>MGSSWSHPQFEKSSGLVPRGSHMLEQCPVTKIGPWGSSHEGTVQDITESPKRLESITLYHGWSVDSISFTYLDHAGEKHKAGPWGGPGGDPIMIEFGSSEFLKEVSGTFGPYEGSTVITSINFITNKQTYGPFGRQEGTPFSVPAQNNSSIVGFFGRSGKYINAVGV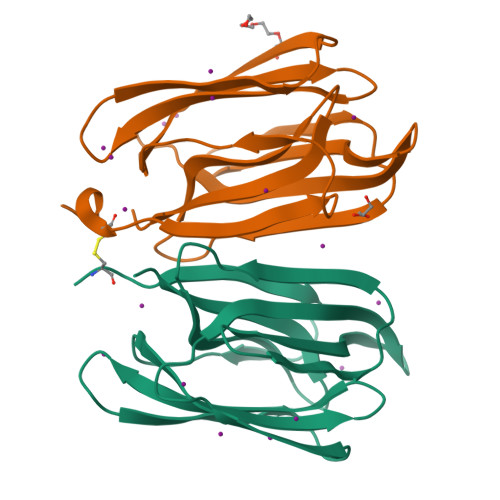YVQPI[2x]>[2x]ADVLNISKIPIFSKKEKKFSDLQKSKEANEKILSKETDRFTLYPILYPDVWDFYKKAEASFWTAEEIDLSSDLKDFEKLNDNEKHFIKHVLAFFAASDGIVLENLASKFLRQVKITEAKKFYAFQIAVENIHSETYSLLIDNYIKDEKERMNLFHAIENIPAVKNKALWAAKWINDTNSFAERIVANACVEGILFSGSFCAIFWFKKQNKLHGLTFSNELISRDEGLH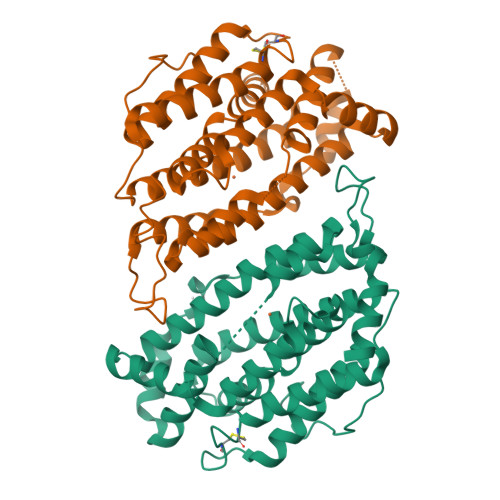TDFNCLIYSLLENKLPEEVVQNIVKEAVEVERSFICESLPCDLIGMNSRLMSQYIEFVADRLLECLGSPKIFHAKNPFNWMDL> ADGGQHWTYEGPHGQDHWPASYPECGNNAQSPIDIQTDSVTFDPDLPALQPHGYDQPGTEPLDLHNNGHTVQLSLPSTLYLGGLPRKYVAAQLHLHWGQKGSPGGSEHQINSEATFAELHIVHYDSDSYDSLSEAAERPQGLAVLGILIEVGETKNIAYEHILSHLHEVRHKDQKTSVPPFNLRELLPK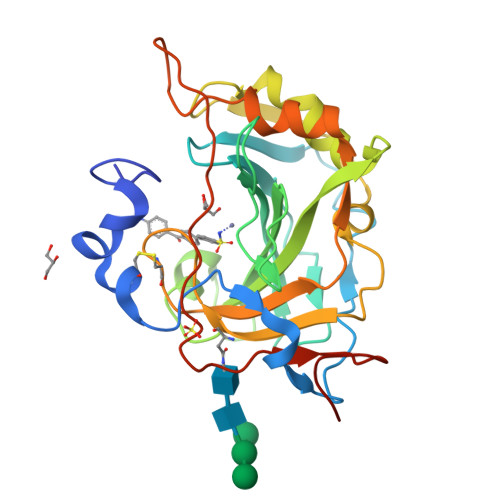QLGQYFRYNGSLTTPPCYQSVLWTVFYRRSQISMEQLEKLQGTLFSTEEEPSKLLVQNYRALQPLNQRMVFASFIQAGSSYTTGEMLVPR> MVHFHPFGNVNFYEMDWSLKGDLWAHAPVIAKEGSRWYVFHTGSGIQIKTSEDGVHWENMGRVFPSLPDWCKQYVPEKDEDHLWAPDICFYNGIYYLYYSVSTFGKNTSVIGLATNRTLDPRDPDYEWKDMGPVIHSTASDNYNAIDPNVVFDQEGQPWLSFGSFWSGIQLIQLDTETMKPAAQAELLTIASRGEEPNA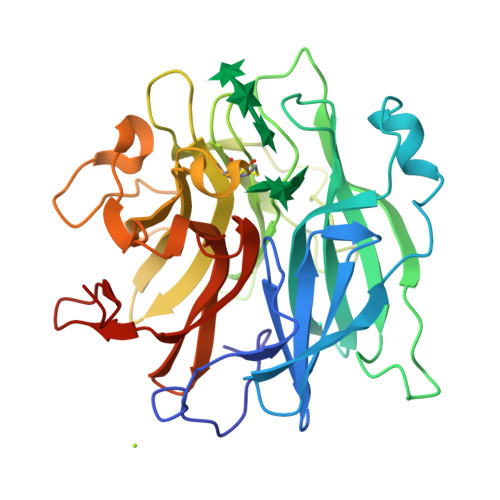IEAPFIVCRNGYYYLFVSFDFCCRGIESTYKIAVGRSKDITGPYVDKNGVSMMQGGGTILDAGNDRWIGPGHCAVYFSGVSAILVNHAYDALKNGEPTLQIRPLYWDDEGWPYLLEHHHHHH>[4x]MNHKVHHHHHHIEGRHMKLAVYSTKQYDKKYLQQVNESFGFELEFFDFLLTEKTAKTANGCEAVCIFVNDDGSRPVLEELKKHGVKYIALRCAGFNNVDLDAAKELGLKVVRVPAYDPEAVAEHAIGMMMTL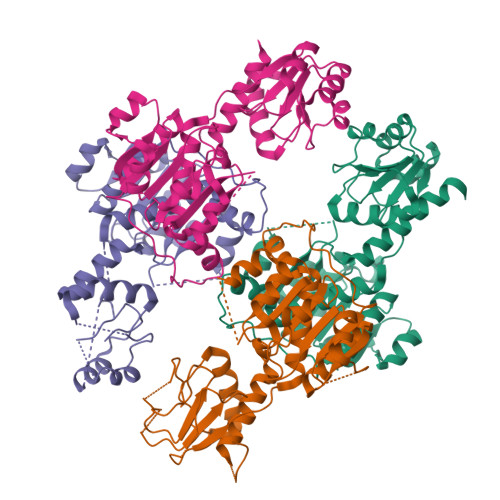NRRIHRAYQRTRDANFSLEGLTGFTMYGKTAGVIGTGKIGVAMLRILKGFGMRLLAFDPYPSAAALELGVEYVDLPTLFSESDVISLHCPLTPENYHLLNEAAFDQMKNGVMIVNTSRGALIDSQAAIEALKNQKIGSLGMDVYENERDLFFEDKSNDVIQDDVFRRLSACHNVLFTGHQAFLTAEALTSISQTTLQNLSNLEKGETCPNELV> MLIQAVGV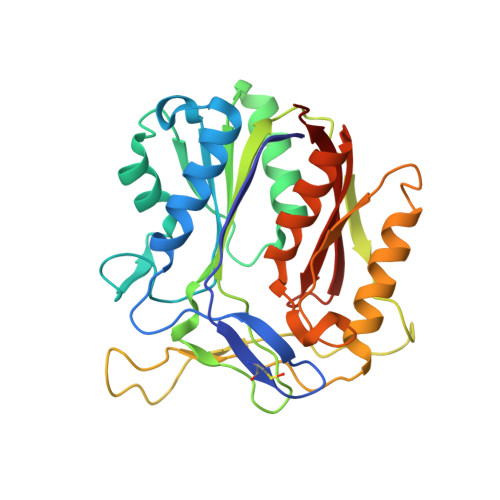NLPPSYVCLEGPLGGERPRAQGDEMLMQRLLPAVREALDEAAVKPEEIDLIVGLALSPDHLIENRDIMAPKIGHPLQKVLGANRAHVFDLTDSSLARALYVVDTLASDQGYRNVLVVRGESSQGLEVDSESGFALADGALALLCRPTGKAAFRRGALGGDPAQEWLPLSIPLNTDIRQVGDVKGHLNLPAQPGLPEAVRAGFTRLAGDFPQLNWVREEWFGQGRPDGRCLGPFELASQLRAAQRDRLDELLLISFDPFGMVVEGVTLELAGEAHA>RSRLTADEYLKIYQAAESSPCWLRLAMELAVVTGQRVGDLCEMKWSDIVDGYLYVEQSKTGVKIAIPTALHIDALGISMKETLDKCKEILGGETIIASTRREPLSSGTVSRYFMRARKASGLSFEGDPPTFHELRSLSARL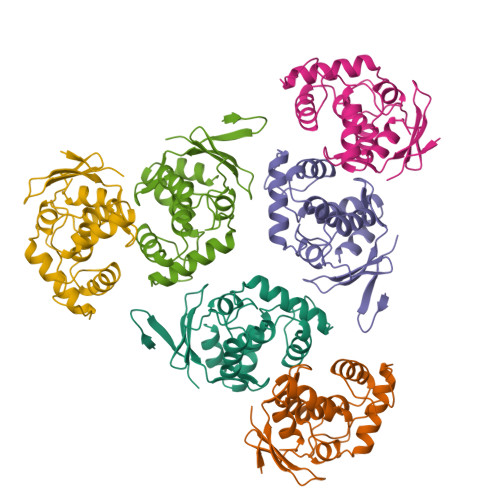YEKQISDKFAQHLLGHKSDTMASQFRDDRGREWDKIEI[2x]>[2x]MED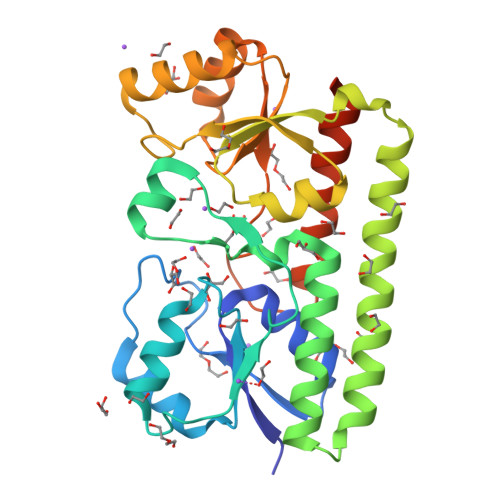GKRLRIGITLHPYYSYVSNIVGDKAEVVPLIPAGFNPGAYEPRAEDIKRIGTLDVVVLNGVGGDDFAERMIASSEKPGIPVIEANAKVPLLAATGMAARGAGKVVNPGTFLSISASITQVNTIARELGKLDPANAKAYTRNARAYAKRLRALRADALARLNKAPAADFRVATIGGAYDYLLREFGLEVTAVVEPAGGIEPSPSQLKKTIDQLKALDVKVIFSEIDFPSTYVETIQRESGVKLYSLSGISYGDYSAGKYEEEMARNLDTVVRAIQESGAENLYFQGHHHHHH3-[(1H-imidazol-1-yl)methyl]-2-phenyl-1H-indole | C18 H15 N3 | 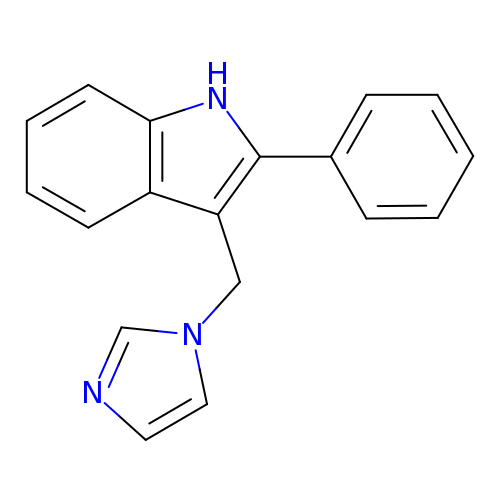RFRCCSUYEPHDFA-UHFFFAOYSA-N>[2x]MSAFDGVENQMNGPDSSPRLSQDPREPRSLLSSSCFPITLKFVDVCYRVKIHGMSNDSCNIKKLLGLKQKPSDETRSTEERTILSGVTGMISPGEFMAVLGPSGSGKSTLLNAVAGRLHGSNLTGKILINDGKITKQTLKRTGFVAQDDLLYPHLTVRETLVFVALLRLPRSLTRDVKLRAAESVISELGLTKCENTVVGNTFIRGISGGERKRVSIAHELLINPSLLVLDEPTSGLDATAALRLVQTLAGLAHGKGKTVVTSIHQPSSRVFQMFDTVLLLSEGKCLFVGKGRDAMAYFESVGFSPAFPMNPADFLLDLA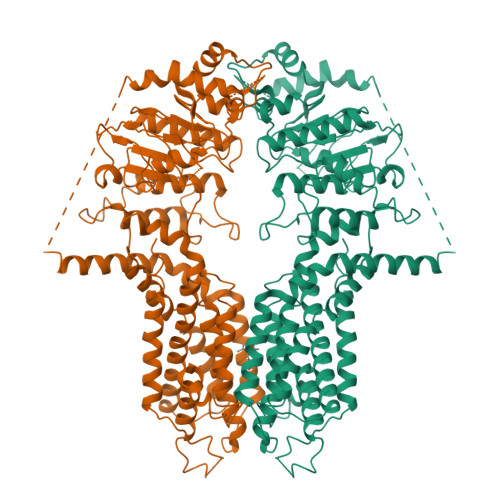NGVCQTDGVTEREKPNVRQTLVTAYDTLLAPQVKTCIEVSHFPQDNARFVKTRVNGGGITTCIATWFSQLCILLHRLLKERRHESFDLLRIFQVVAASILCGLMWWHSDYRDVHDRLGLLFFISIFWGVLPSFNAVFTFPQERAIFTRERASGMYTLSSYFMAHVLGSLSMELVLPASFLTFTYWMVYLRPGIVPFLLTLSVLLLYVLASQGLGLALGAAIMDAKKASTIVTVTMLAFVLTGGYYVNKVPSGMVWMKYVSTTFYCYRLLVAIQYGSGEEILRMLGCDSKGKQGASAATSAGCRFVEEEVIGDVGMWTSVGVLFLMFFGYRVLAYLALRRIKH> MSSNRVLDLFKPFESFLPEVIAPERKVPYNQKLIWTGVSLLIFLILGQIPLYGIVSSETSDPLYWLRAMLASNRGTLLELGVSPIITSSLIFQFLQGTQLLQIRPESKQDRELFQIAQKVCAIILILGQALVVVMTGNYGAPSDLGLPICLLLIFQLMFASLIVMLLDELLSKGYGLGSGISLFIATNIAEQIFWRAFAPTTVNSGRGKEFEGAVIAFFHLLAVRKDKKRALVEAFYRTNLPNMFQVLMTVAIFLFVLYLQGFRYELPIRSTKVRGQIGIYPIKLFYTSNTPIILQSALTSNIFLISQILFQKYPTNPLIRLIGVWGIRPGTQGPQMALSGLAYYIQPLMSLSEALLDPIKTIVYITFVLGSCAVFSKTWIEISGTSPRDIAKQFKDQGMVINGKRETSIYRELKKIIPTAAAFGGATIGALSVGSDLLGTLGSGASILLATTTIYGYYEAAAKEGGFTKNLVPGFSDLM;> MSSPTPPGGQRTLQKRKQGSSQKVAASAPKKNTNSNNSILKIYSDEATGLRVDPLVVLFLAVGFIFSVVALHVISKVAGKLF;> MARASEKGEEKKQSNNQVEKLVEAPVEFVREGTQFLAKCKKPDLKEYTKIVKAVGIGFIAVGIIGYAIKLIHIPIRYVIV;> PTNYEYDEASETWPSFILTGLLMVVGPMTLLQIYQIFFGANAEDGNSGKSKEFNEEVFKNLNEEYTSDEIKQFRRKFDKNSNKKSKIWSRRNIIIIVGWILVAILLQRINSNDAIKDAATKLFDPYEILGISTSASDRDIKSAYRKLSVKFHPDKLAKGLTPDEKSVMEETYVQITKAYESLTDELVRQNYLKYGHPDGPQSTSHGIALPRFLVDGSASPLLVVCYVALLGLILPYFVSRWWARTQSYTKKGIHNVTASNFVSNLVNYKPSEIVTTDLILHWLSFAHEFKQFFPDLQPTDFEKLLQDHINRRDSGKLNNAKFRIVAKCHSLLHGLLDIACGFRNLDIALGAINTFKCIVQAVPLTPNCQILQLPNVDKEHFITKTGDIHTLGKLFTLEDAKIGEVLGIKDQAKLNETLRVASHIPNLKIIKADFLVPGENQVTPSSTPYISLKVLVRSAKQPLIPTSLIPEENLTEPQDFESQRDPFAMMSKQPLVPYSFAPFFPTKRRGSWCCLVSSQKDGKILQTPIIIEKLSYKNLNDDKDFFDKRIKMDLTKHEKFDINDWEIGTIKIPLGQPAPETVGDFFFRVIVKSTDYFTTDLDITMNMKVRDSPAVEQVEVYSEEDDEYSTDDDETESDDESDASDYTDIDTDTEAEDDESPE;> MSEFNETKFSNNGTFFETEEPIVETKSISVYTPLIYVFILVVSLVMFASSYRKKQAKKISEQPSIFDENDAHDLYFQIKEMSENEKIHEKVLKAALLNRGAESVRR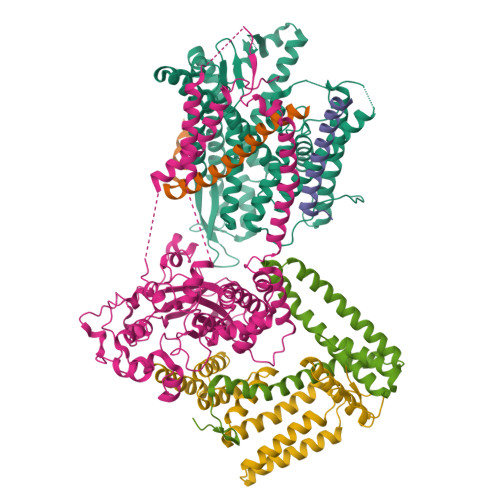SLKLKELAPQINLLYKNGSIGEDYWKRFETEVKLIELEFKDTLQEAERLQPGWVQLFVMVCKEICFNQALSRRYQSILKRKEVCIKEWELKINNDGRLVN;> MVTLEYNANSKLITASDAVVALSTETNIDQINVLTTSLIGETNPNFTPQPNEALSKMIKGLFESGMKNLQQKKLNEALKNVSLAIEMAQRKRAPWEAFAIQLPELHFMLRSKIDLCLILGKHLEALQDLDFLLGTGLIQPDVFVRKADCLLKLRQWEEARATCERGLALAPEDMKLRALLIETARNLAEYNGE>[4x]MPRRDRNMDSAPCMWMRGGTSKGGYFLRADLPADTAARDAFLLAVMGSPDPRQIDGMGGADPLTSMVAVVSKSERPGIDVDYLFLQVFVDQAIVTDAQNCGNILAGVGPFAIERGLVAASGDETRVAIFMENTGQVAVATVRTPGGSVTYAGDAAIDGVPGTHAPIPTEFRDTAGSSCGALLPSGNAVDVVNGLPVTLIDNGMPCVVMKAADVGITGYEDRDSLDANAELKAKIEAIRLAVG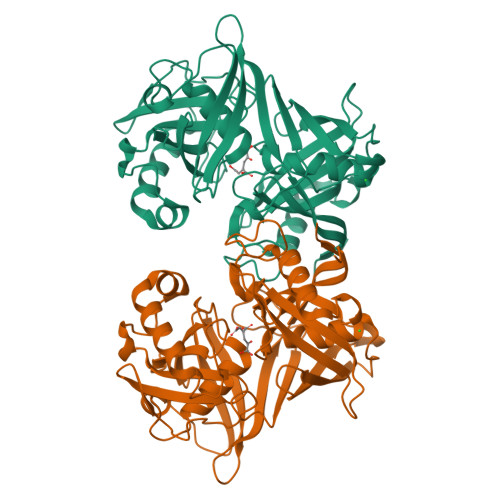ELMNLGDVTEKSVPKMMLVAPPRDGGAVCVRSFIPHRAHATIGVLGAVSVATACLIPGSPAAEVAVVPEGARKTLSIEHPTGEMSCVLEVDDAGNVVSAALLRTARKLMDGVVFVLEHHHHHH>TINKSHDVVIIGGGPAGYVAAIKAAQLGFNTACVEKRGKLGGTCLNVGCIPSKALLNNSHLFHQMHTEAQKRGIDVNGDIKINVANFQKAKDDAVKQLTGGIELLFKKNKVTYYKGNGSFEDETKIRVTPVDGLEGTVKEDHILDVKNIIVATGSEVTPFPGIEIDEEKIVSSTGALSLKEIPKRLTIIGGGIIGLEMGSVYSRLGSKVTVVEFQPQIGASMDGEVAKATQKFLKKQGLDFKLSTKVISAKRNDDKNVVEIVVEDTKTNKQENLEAEVLLVAVGRRPYIAGLGAEKIGLEVDKRGRLVIDDQFNSKFPHIKVVGDVTFGPMLA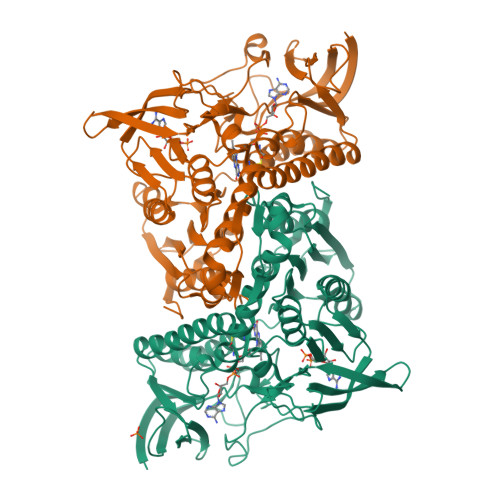HKAEEEGIAAVEMLKTGHGHVNYNNIPSVMYSHPEVAWVGKTEEQLKEAGIDYKIGKFPFAANSRAKTNQDTEGFVKILIDSKTERILGAHIIGPNAGEMIAEAGLALEYGASAEDVARVCHAHPTLSEAFKEANMAAYDKAIHC[2x]Transcription factors (TFs) recognize specific bases within their DNA-binding motifs, with each base contributing nearly independently to total binding energy. However, the energetic contributions of particular dinucleotides can deviate strongly from the additive approximation, indicating that some TFs can specifically recognize DNA dinucleotides. Here we solved high-resolution (<1 Å) structures of MYF5 and BARHL2 bound to DNAs containing sets of dinucleotides that have different affinities to the proteins. The dinucleotides were recognized either enthalpically, by an extensive water network that connects the adjacent bases to the TF, or entropically, by a hydrophobic patch that maintained interfacial water mobility.

We first assessed whether differences in resolution would affect the detection of the water molecules using the two BARHL2–DNAAC structures solved at 0.95 Å and 1.3 Å. Although overall more water molecules are seen in the protein–DNA interface in the 0.95 Å structure, inspection of the water content at the site of the variant dinucleotide at both resolutions showed conserved positions of all of the ten water molecules, indicating that at this range, resolution does not substantially affect detection of water molecules contributing to recognition of the dinucleotide. Analysis of the highest-affinity complex, BARHL2–DNAAC, revealed that the high-affinity binding of BARHL to DNAAC is caused by a combination of indirect and direct recognition of DNA. Key amino acids involved in the recognition of the AC dinucleotide and its complementary bases are Asn282 and two threonines: Thr278 and Thr285. Thus, Thr278 orders water molecules in such a way that they contact both bases of the AC dinucleotide. The T18 opposite to the A7 of the AC dinucleotide is also recognized directly by a hydrophobic contact to the methyl group (CG2) of Thr285. In addition, the side-chain oxygen of Thr285 contacts N7 of the G17 opposite to the AC dinucleotide through a water molecule that is a part of the second water chain. Most of the low-entropy waters form a stable hydrogen bond network connecting the recognition helix of BARHL2 with bases at the TAAAC site, in good agreement with the water molecules observed in the two BARHL2–DNAAC structures resolved at 0.95 Å and 1.3 Å. The strongly localized and extensive water network that connects BARHL2 amino acids to the AC dinucleotide is enthalpically favorable for binding but entropically unfavorable.

> PRKARTAFSDHQLNQLERSFERQKYLSVQDRMDLAAALNLTDTQVKTWYQNRRTKWKRQTAV N-[3-(azepan-1-yl)propyl]-5-methyl-4-oxo-4,5-dihydrothieno[3,2-c]quinoline-2-carboxamide 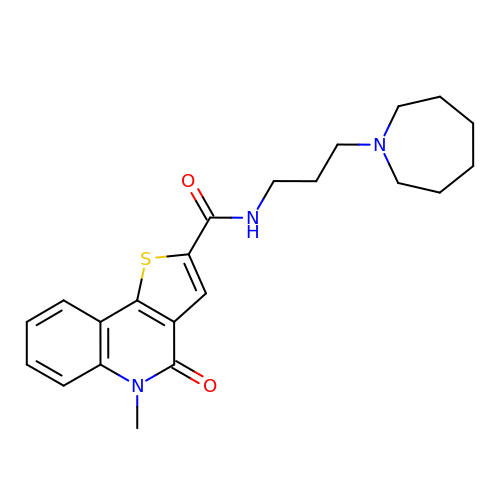| C22 H27 N3 O2 S | NVFMMXVDSJFVNO-UHFFFAOYSA-N> E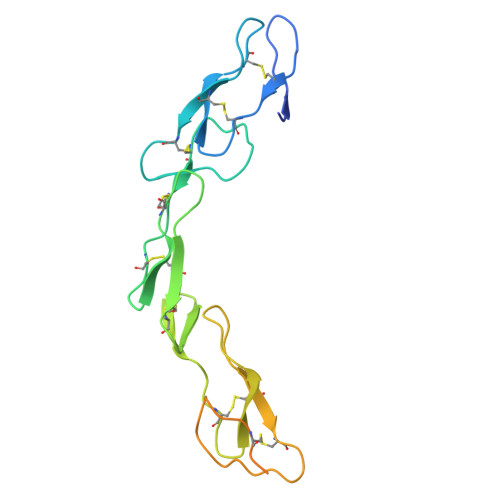TLPPKYLHYDPETGHQLLCDKCAPGTYLKQHCTVRRKTLCVPCPDHSYTDSWHTSDECVYCSPVCKELQSVKQECNRTHNRVCECEEGRYLEIEFCLKHRSCPPGSGVVQAGTPERNTVCKKCPDGFFSGETSSKAPCIKHTNCSTFGLLLIQKGNATHDNVCSGNREATQKCGIASSVLPR> GHMSSDIDELRREIDIVDVISEYLNLEKVGSNYRTNCPFHPDDTPSFYVSPSKQIFKCFGCGVGGDAIKFVSLYEDISYFEAALELAKRYGKKLDLEKISKDEKVYVALDRVCDFYRESLLKNREASEYVKSRGIDPKVARKFDLGYAPSSEALVKVLKENDLLEAYLETKNLLSPTKGVYRDLFLRRVVIPIKDPRGRVIGFGGRRIVEDKSPKYINSPDSRVFKKGENLFGLYEAKEYIKEEGFAILVEGYFDLLRLFSEGIRNVVAPLGTALTQNQANLLSKFTKKVYILYDGDDAGRKAMKSAIPLLLSAGVEVYPVYLPEGYDPDEFIKEFGKEELRRLINSSGELFETLIKTARE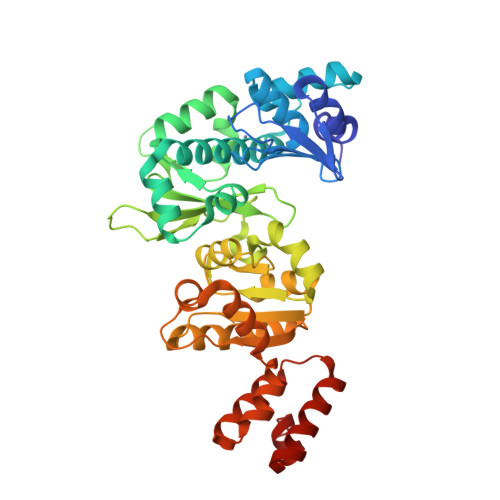NLEEKTREFRYYLGFISDGVRRFALASEFHTKYKVPMEILLMKIEK>[8x]ADKLPYKVADIGLAAWGRKALDIAENEMPGLMRMREMYSASKPLKGARIAGCLHMTVETAVLIETLVALGAEVRWSSCNIFSTQDHAAAAIAKAGIPVFAWKGETDEEYLWCIEQTLHFKDGPLNMILDDGGDLTNLIH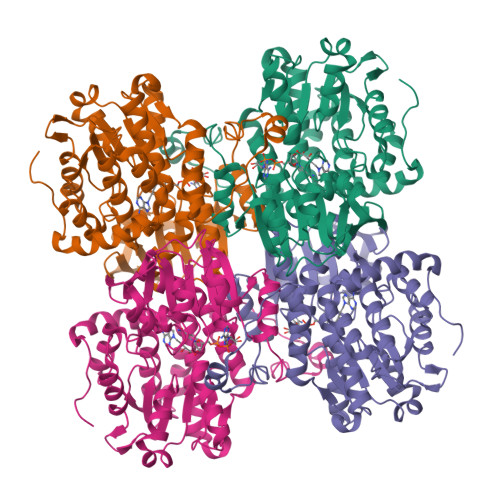TKHPQLLSGIRGISEETTTGVHNLYKMMANGILKVPAINVNDSVTKSKFDNLYGCRESLIDGIKRATDVMIAGKVAVVAGYGDVGKGCAQALRGFGARVIITEIDPINALQAAMEGYEVTTMDEACKEGNIFVTTTGCVDIILGRHFEQMKDDAIVCNIGHFDVEIDVKWLNENAVEKVNIKPQVDRYLLKNGHRIILLAEGRLVNLGCAMGHPSFVMSNSFTNQVMAQIELWTHPDKYPVGVHFLPKKLDEAVAEAHLGKLNVKLTKLTEKQAQYLGMPINGPFKPDHYRY>TATYSGNPFVGVTPWANAYYASEVSSLAIPSLTGAMATAAAAVAKVPSFMWLDTLDKTPLMEQTLADIRTANKNGGNYAGQFVVYDLPDRDCAALASNGEYSIADGGVAKYKNYIDTIRQIVVEYSDIRTLLVIEPDSLANLVTNLGTPKCANAQSAYLECINYAVTQLNLPNVAMYLDAGHAGWLGWPANQDPAAQLFANVYKNASSPRALRGLATNVANYNGWNITSPPSYTQGNAVYNEKLYIHAIGPLLANHGWSNAFFITDQGRSGKQPTGQQQWGDWCNVIGTGFGIRPSANTGDSLLDSFVWVKPGGECDGTSDSSAPRFDSHCALPDALQ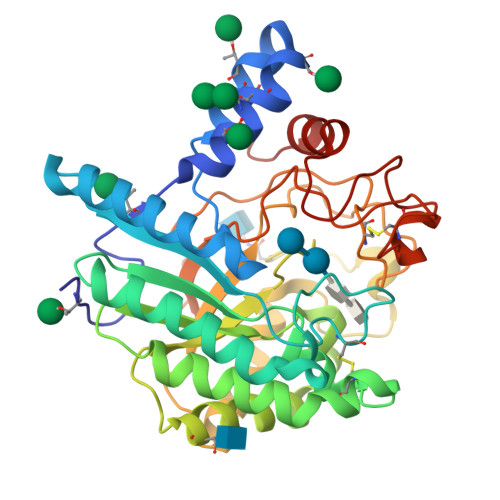PAPQAGAWFQAYFVQLLTNANPSFL[2x]> MAAADGDDSLYPIAVLIDELRNEDVQLRLNSIKKLSTIALALGVERTRSELLPFLTDTIY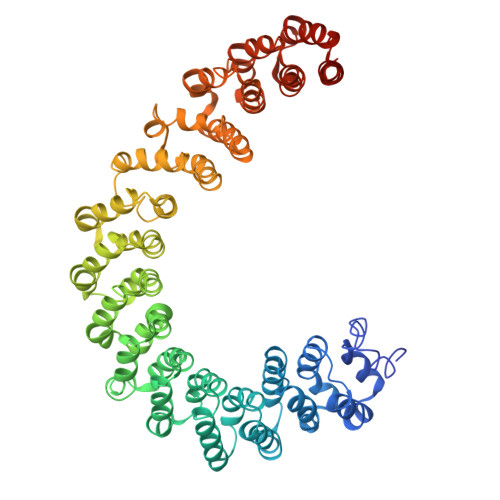DEDEVLLALAEQLGTFTTLVGGPEYVHCLLPPLESLATVEETVVRDKAVESLRAISHEHSPSDLEAHFVPLVKRLAGGDWFTSRTSACGLFSVCYPRVSSAVKAELRQYFRNLCSDDTPMVRRAAASKLGEFAKVLELDNVKSEIIPMFSNLASDEQDSVRLLAVEACVNIAQLLPQEDLEALVMPTLRQAAEDKSWRVRYMVADKFTELQKAVGPEITKTDLVPAFQNLMKDCEAEVRAAASHKVKEFCENLSADCRENVIMTQILPCIKELVSDANQHVKSALASVIMGLSPILGKDNTIEHLLPLFLAQLKDECPEVRLNIISNLDCVNEVIGIRQLSQSLLPAIVELAEDAKWRVRLAIIEYMPLLAGQLGVEFFDEKLNSLCMAWLVDHVYAIREAATSNLKKLVEKFGKEWAHATIIPKVLAMSGDPNYLHRMTTLFCINVLSEVCGQDITTKHMLPTVLRMAGDPVANVRFNVAKSLQKIGPILDNSTLQSEVKPILEKLTQDQDVDVKYFAQEALTVLSLA>MEDMILTEEMQKIMNLIQDDENNVFVTGKAGSGKTTFLKYLIEKSGKNCIVAAPTGIAAINAGGVTLHSLFGIPFGPITPYDRLENKFSEYKVELLLKMELLIIDEISMVRPDILDTIDRKLRWVYESDEPFGGVQVVMFGDLFQLPPVTKKQEREILSDFYDGFFFFNALVFKRTGFHIVELTKIFRQTEPEFINVLNNIRNYQVTSDELDLLSELKDRKISSSYDNEYIHICTHKADVEKINADKLGEQEIRNYDIVIKDKFPESSIPCDLHLKLRVGARVMSLVNDSLKGYYNGMLGIVTALEDNVITVRMDNGRTIKFERYTWSNTQYTLKDNEIVKEEIGSCTQFPLTLAWAITIHKSQGLTFDKIIIHVSHTF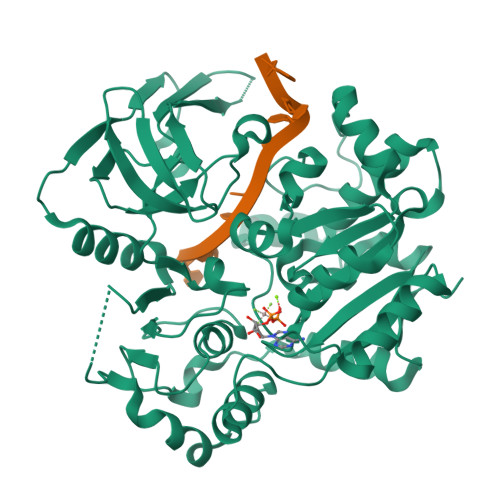CPGQLYVALSRCRTLEGIVSDAFITKQMIIPEYALIDFERAYKSEGNYYGKRLD[2x]>GYSCRAVGVDGRAVTDIQGTCHAKATGAGAMASGTSEPGS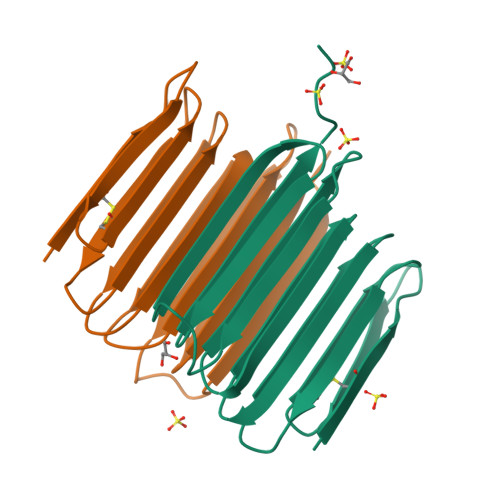TSTATATGRGATARSTSTGRGTATTTATGTASATSNAIGQGTATTTATGSAGGRATGSATTSSSASQPTQTQTITGPGFQTAKSFARNTATTTVTASHHHHHH[2x]>[2x]MKYRCKVCDYIYDPEVGDPTSGIKPGTPFQELPEDWLCPVCNVGKDQFEPLRGEVRRVRPEDIDMFYYQCSQTVRGRACTVKGVCGKEATVARLQDNLLFAIKGISAYLYHARELGYTDEVVDAFLERGFYSTLTNVNFDAEEFVSLALEAGEMNLRTMKLLKKAHMDTYGEPEPAEVRVGALDGPAIIATGHSLKALEELLKQTEGSGVNVYTHSELLPAHGYPGLRKYPHLAGQLGGPWFDQRETFSRYSAAVLGTSNCVLLPRDSYRDRMFTCGVARLPGVEHVDGYDFSPVIEKALELPPLKEEDSATLTTGFGLSTILSLADKIKELVEEGKIRRFFLVGGCDSPLPQAKYYTEFVRKLPEDTVVLTLACGKYRFNSMDLGDIDGIPRLIDLGQCNDSIVAVELVEALSNLFSMDVNELPLSIVLSWMEQKAAAILWSLLSLNLRGMYIGPILPGWANDDIINVLVDKYELTPIGDPEEDIKKMMEVDKLAAALEHHHHHH

Hybrid cluster proteins (HCPs) are unique Fe-S-O-type metallocluster (hybrid cluster)-containing enzymes. They play key roles in nitrogen metabolism, stress responses and protein S-nitrosylation in microorganisms under anaerobic conditions. Hybrid cluster proteins (HCPs) are Fe-S-O cluster-containing metalloenzymes in three distinct classes (class I and II: monomer, III: homodimer), all of which structurally related to homodimeric Ni, Fe-carbon monoxide dehydrogenases (CODHs). Here we show X-ray crystal structure of class III HCP from Methanothermobacter marburgensis (Mm HCP), demonstrating its homodimeric architecture structurally resembles those of CODHs.

The crystal structure of Mm HCP C67Y was determined at 3.0 Å resolution. This variant exhibited a homodimeric architecture identical to that of Mm HCP wild-type (WT), demonstrating the rigidity of the dimeric architecture. However, no electron density maps of rubredoxin and the [4Fe-4S] cluster-binding domains of Mm HCP C67Y were observed. This indicates that these regions were disordered, which could have been caused by the lack of the Cys ligand at position 67 in the [4Fe-4S] cluster. In Mm HCP C67Y, Glu434 was positioned at the solvent-exposed area, far from the hybrid cluster, although Glu434 of WT is a ligand of the hybrid cluster. Superimposing Mm HCP WT and C67Y showed that the regions around Glu434 and Trp461 were shifted by ~5.3–5.8 Å. Owing to the denaturation, the loop region around Glu434 became unstabilized and shifted to the solvent area, which may have been favourable because the hydrophilic residues, including Glu434, may compensate for the positions where the [4Fe-4S] cluster-binding domain of WT was occupied, resulting in the stabilisation of this area via networks of polar interactions with solvent waters. Mm HCP C67S and C67Y were less active than WT, as they exhibited lower kcat and higher KM values than WT. Considering similar spectral features of Mm HCP C67S and C67Y variants and the structure of Mm HCP C67Y, the lower activity was caused by the fact that Mm HCP C67S and C67Y variants had neither [4Fe-4S] cluster nor Glu-coordination to the hybrid cluster.> GSHMQDPEQLKHCNGILKELLSSKHAAYAWPFYKPVDASALGLHDYHDIIKHPMDL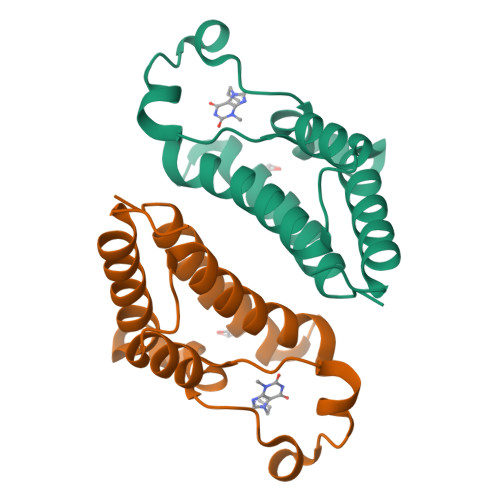STVKRKMENRDYRDAQEFAADVRLMFSNCYKYNPPDHDVVAMARKLQDVFEFRYAKMPD> MSYHNHNHNHNHNHNDYDIPTTENLYFQGAMDLMPPGVDCPMEFWTKEESQSVVVDFLLPTGVYLNFPVSRNANLSTIKQVLWHRAQYEPLFHMLSDPEAYVFTCVNQTAEQQELEDEQRRLCDIQPFLPVLRLVAREENLYFQGGDRVKKLINSQISLLIGKGLHEFDSLRDPEVNDFRTKMRQFCEEAAAHRQQLGWVEWLQYSFPLQLEPSARGWRAGLLRVSNRALLVNVKFEGSEESFTFQVSTKDMPLALMACALRKKATVFRQPLVEQPEEYALQVNGRHEYLYGNYPLCHFQYICSCLHSGLTPHLTMVHSSSILAMRDEQSNPAPQVQKPRAKPPPIPAKKPSSVSLWSLEQPFSIELIEGRKVNADERMKLVVQAGLFHGNEMLCKTVSSSEVNVCSEPVWKQRLEFDISVCDLPRMARLCFALYAVVEKAKKARSTKKKSKKADCPIAWANLMLFDYKDQLKTGERCLYMWPSVPDEKGELLNPAGTVRGNPNTESAAALVIYLPEVAPHPVYFPALEKILELGRHGERGRITEEEQLQLREILERRGSGELYEHEKDLVWKMRHEVQEHFPEALARLLLVTKWNKHEDVAQMLYLLCSWPELPVLSALELLDFSFPDCYVGSFAIKSLRKLTDDELFQYLLQLVQVLKYESYLDCELTKFLLGRALANRKIGHFLFWHLRSEMHVPSVALRFGLIMEAYCRGSTHHMKVLMKQGEALSKLKALNDFVKVSSQKTTKPQTKEMMHMCMRQETYMEALSHLQSPLDPSTLLEEVCVEQCTFMDSKMKPLWIMYSSEEAGSAGNVGIIFKNGDDLRQDMLTLQMIQLMDVLWKQEGLDLRMTPYGCLPTGDRTGLIEVVLHSDTIANIQLNKSNMAATAAFNKDALLNWLKSKNPGEALDRAIEEFTLSCAGYCV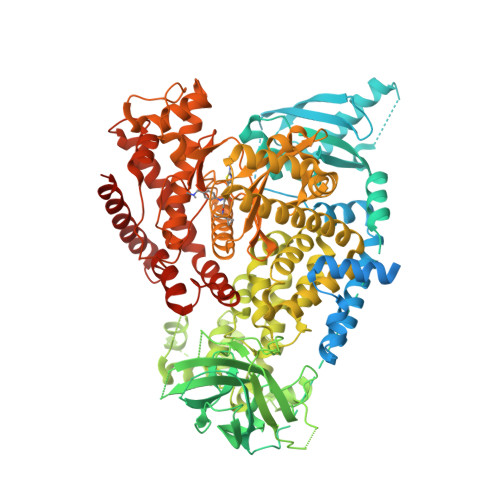ATYVLGIGDRHSDNIMIRESGQLFHIDFGHFLGNFKTKFGINRERVPFILTYDFVHVIQQGKTNNSEKFERFRGYCERAYTILRRHGLLFLHLFALMRAAGLPELSCSKDIQYLKDSLALGKTEEEALKHFRVKFNEALRESWKTKVNWLAHNVSKDNRQ> KPAAHLIGDPSKQNSLLWRANTDRAFLQDGFSLSNNSLLVPTSGIYFVYSQV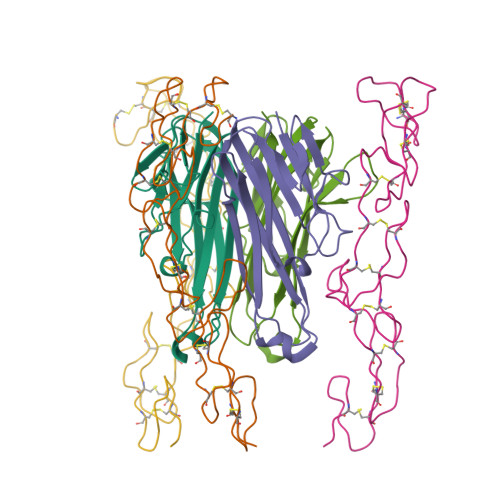VFSGKAYSPKATSSPLYLAHEVQLFSSQYPFHVPLLSSQKMVYPGLQEPWLHSMYHGAAFQLTQGDQLSTHTDGIPHLVLSPSTVFFGAFAL;> CPQGKYIHPQNNSICCTKCHKGTYLYNDCPGPGQDTDCRECESGSFTASENHLRHCLSCSKCRKEMGQVEISSCTVDRDTVCGCRKNQYRHYWSENLFQCFNCSLCLNGTVHLSCQEKQNTVCTCHAGFFLRENECVSC> KESRAKAFQRQHMDSDSSPSSSSTYCNQMMRRRNMTQGRCKPVNTFVHEPLVDVQNVCFQEKVTCKNG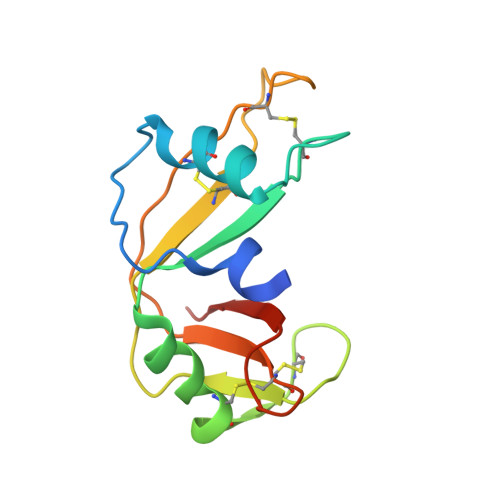QGNCYKSNSSMHITDCRLTNGSRYPNCAYRTSPKERHIIVACEGSPYVPVHFDASVEDST PB1 domains are protein interaction modules with critical roles in the assembly of protein complexes involved in autophagy, signaling, cell division, and redox processes, as well as the auxin-response pathway in plants. PB1 domains form homotypic interactions via conserved electrostatic motifs molded by basic or acidic surface patches on opposite faces of their ubiquitin-like β-grasp fold. While type A and type B PB1 domains can form heterodimeric protein complexes, type AB members can mediate interactions with either PB1 domain type or engage in homotypic interactions to form homo-oligomers or hetero-oligomers. Our cryo-EM structures of filamentous p62 and AtNBR1–PB1 assemblies revealed that the presence of a tandem arginine sequence in the basic motif of type AB interfaces is required to stabilize a polymeric assembly.

Of the three PB1 assemblies studied, AtNBR11–94 (AtNBR1–PB1) and p621–122 (p62-PB1) formed homogeneous filaments of constant diameter that appeared best suited for high-resolution structure investigation by cryo-EM. Image classification of segmented PB1 helices revealed that both AtNBR1–PB1 and p62-PB1 polymerize in two different tubular morphologies: a projection class with a ladder-like pattern, we term L-type, and a projection class with a serpent-like one, we term S-type. Further analysis revealed that the occurrence of L-type or S-type assemblies is persistent along the individual helices in micrographs of AtNBR1–PB1, whereas for p62-PB1 filaments regularly displayed transitions from L-type to S-type symmetry. By indexing the layer lines in the Fourier spectra of AtNBR1–PB1 filaments, we concluded that L-type is a two-stranded helix with a pitch of 77.2 Å and 11.47 subunits/turn, whereas S-type is a single double-stranded helix with a pitch of 68.2 Å and 11.55 subunits/turn. Using the derived symmetries, we determined the 3.5/3.9- (L-type, p62/AtNBR1) and 4.0/4.4 Å- (S-type, p62/AtNBR1) resolution structures. All four structures form tubules of ~120 Å and 150-Å width with an inner diameter of 45 Å and 70 Å for AtNBR1–PB1 and p62-PB1, respectively. The relative orientation between adjacent subunits is very similar in the respective S-type and L-type assemblies of AtNBR1–PB1 and p62-PB1. The main interactions are formed between a double arginine finger formed by two neighboring arginine residues in strand β2 (R19–R20AtNBR1/R21–22p62) stabilizing strong salt bridges to acidic residues (D60/D62/D64/D73AtNBR1 or D69/D71/D73/E82p62) in the OPCA motif located in the β2–β3 loop and the α2 helix. These interactions are assisted by the canonical-type B lysine (K11AtNBR1 and K7p62) in strand β1. In addition to the canonical transverse interactions, the helices are further stabilized by longitudinal interactions Y14AtNBR1/N28AtNBR1 or K102p62/D92p62 and R59p62/D93p62 to subunits of neighboring strands along the helical axis.

>[2x]MESTANALVVKVSYGGVLRRFRVPVKANGQLDLEMAGLKEKIAALFNLSADAELSLTYSDEDGDVVALVDDNDLFDVTNQRLKFLKINVNAGVS> MTKAIPWKINWQTMAFEYIGPQIEALLGWPQGSWKSVEDWATRMHPEDQEWVVNFCVKQSECGVDHEADYRALHRDGHYVWIRDVVHVVRD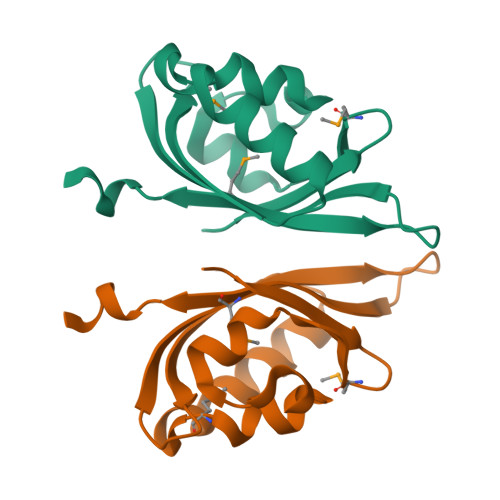DSGEVEALIGFMFDISLEHHHHHH>[2x]SNAMLLYTKKDDIYSDIVRMILLIKGANAKIVDVSKEENSKHLEELNIITPNGNIPTLSTDDFAVYRLSVIIEAIEDLYPFPPMFPVFPKQRANARILLEYVNKTFLQNIIKL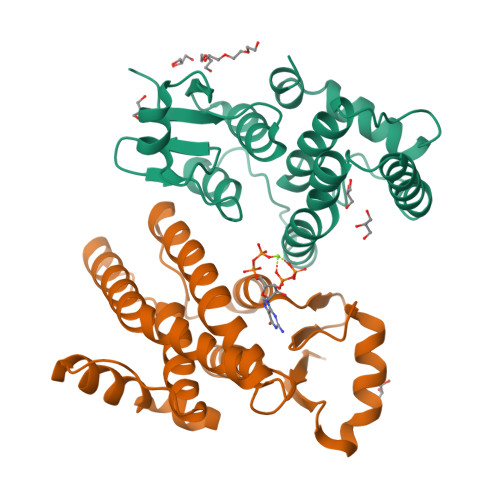QSPDLDEKQANEIKMLMQRDIISTYKKIVSEREVNAESNPDAQNINVLTLIITFVFYYFIKLKISIPTKDKNIIKEIKELLSEPNFIKTIK;>[2x]SNAMVTLYTTKYCPYSLRARIALAEKKMSTDIVEAGDLEPAMIKKITPNGVFPVLMEKDYSINNRKALLIYIDERFPAPSLLPNVVNERIKIRLSLDKIDNEWYPVLDQIRKHRSDQKMLESMFKDLKESLLAMEKAFTGSEFFISSGFTLADCYIAALIICLEAEGFIIDDEYGAIYEYKKRLFARDSVKKANIKGGAGESLLKTLRTHR> MDAEEKMGVELSSPSAIMEHARRLYMSKDYRSLESLFGRCLWKSYNLDLWMLYIEYVRKVSQKKFKLFEVYEFTLGQFENYWDSYGLFKEYIEELGKIEDEQTRIEKIRNGYMRALQTPMGSLSELWKDFENFELELNKITGKKIVGDTLPLFQSSFQRYQQIQPLIRGWSVKNAARLIDLEMENGMKLGGRPHESRMHFIHNYILDSFFYAEEVYFFYSEYLIGIGQKEKAKKVVERGIEMSDGMFLSLYYGLVMDEEAVYGDLKRKYSMGEAESAEKVFSKELDLLRINHLNYVLKKRGLELFRKLFIELGNEGVGPHVFIYCAFIEYYATGSRATPYNIFSSGLLKHPDSTLLKEEFFLFLLRIGDEENARALFKRLEKTSRMWDSMIEYEFMVGSMELFRELVDQKMDAIKADAILPPLPPREHNVQMEGILGRYHCFLDSFNFLDLKIR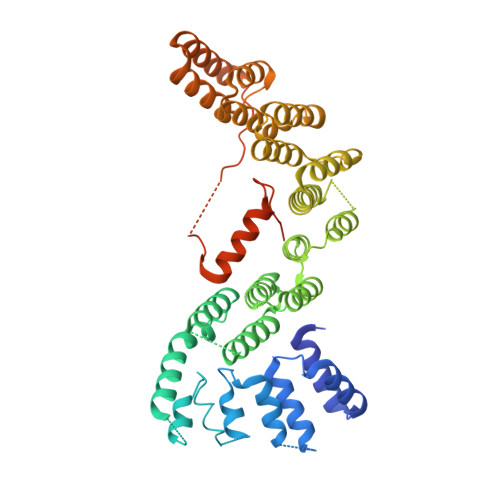DNSRLLDEFMENLPKISQQNNVLSNLRVEKVISLLKSVQ>GSHMRSLESLHSFVAAATKELMWLNEKEEEEVGFDWSDRNTNMTAKKESYSALMRELELKEKKIKELQNAGDRLLREDHPARPTVESFQAALQTQWSWMLQLCCCIEAHLKENAAYFQFFSDVREAEGQLQKLQEALRRKYSCDRS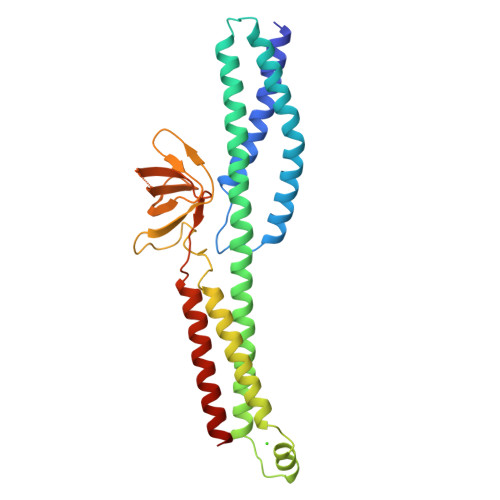ATVTRLEDLLQDAQDEKEQLNEYKGHLSGLAKRAKAVVQLKPRHPAHPMRGRLPLLAVCDYKQVEVTVHKGDECQLVGPAQPSHWKVLSSSGSEAAVPSVCFLVPPPNQEAQEAVTRLEAQHQALVTLWHQLHVDMK[2x]> MGSSHHHHHHSSGRENLYFQGHMREHLKLFSLIFSYPDEDKLGKAIALAEGIGLTEIAQTLKQVDIEALQVEYTSLFISSHPSVPCPPYQSYFEEGSVYGKASLRAAELYSKYGLNYVYESEPPDHISVELEFLSMNPELLSDFRDWFLEFAKCVEEKSEIYATFA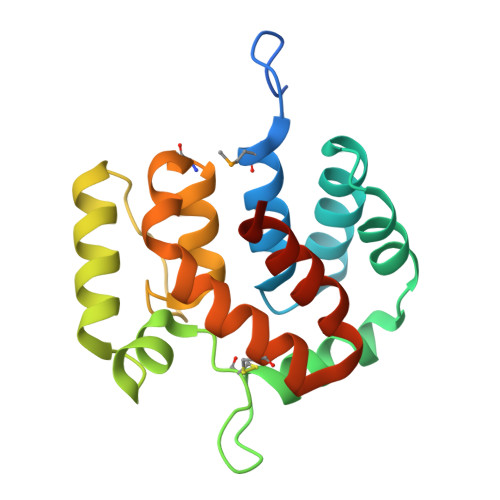RAFRKFLEKPSKVQS AvaII from the filamentous cyanobacterium Anabaena variabilis has attracted our interest because it exhibits robust activity against the RNA and DNA strands of an RNA/DNA heteroduplex. As most other enzymes with such properties, AvaII is a Type II restriction endonuclease predicted to belong to the PD-(D/E)XK superfamily. The enzyme is specific for DNA with the G↓GWCC sequence (where W stands for an A or T base of a ‘weak’ base pair) and cleaves it to products with three nucleotide long 5′-overhangs. The core of the AvaII protomer adopts the same conformation in all three structures, and consists of the characteristic αββββ motif of the PD-(D/E)XK endonucleases.

A ‘closed’ conformation is observed in the complex of AvaII with partially cleaved dsDNA. In the closed complex, the DNA is bound to the enzyme by a set of base specific as well as backbone interactions. Moreover, the catalytic sites are optimally positioned in the close vicinity of the partially cleaved phosphoester bonds. We therefore interpret this complex as specific. In contrast, dsDNA was partially cleaved, due to either trace amounts of Mg2+ ions in the crystallization mix (resulting from reagent impurities), or the presence of Ca2+ ions and the long time for crystallization (9 months). In the specific complex of AvaII with dsDNA, the attacking water molecule (hydroxide ion) is either partially or fully incorporated into the reaction product. To our surprise, instead of an amino acid in this region, we found density for a central octahedrally coordinated atom with six solvent molecule ligands. Ligand locations and distances of around 2.2 Å suggested that the ion should be interpreted as Ca2+. Irrespective of the physiological identity of the metal ion, it is likely responsible for the preference for W over S in the central position. In summary, we conclude that there is strong evidence that AvaII binds dsDNA in the A-like conformation.

>[2x]MGSKFIQNAAEIAKKAMDSVDPSLSEKFTIVIRFLTDNPDAASALKGKERSIVGTEEYIIASATNFKKGRDPRTPLPPSTIPDEMVSVILNKYFEVPSEELEKAEEWHRLSMGAENIVGDLLERYIAEVIEPHGWIWCSGSMVRAVDFIYCDSENVWQSLQVKNRDNTENSSSAAIRHGTPIKKWFRTFSKKRGDNWDKFPSLEGKENLSEKGFKLYVEKYLSALRAIKALEHHHHHH4-{[6-(cyclohexylmethyl)pyridine-2-carbonyl]amino}-3-[(4-fluorophenyl)amino]benzoic acid | C26 H26 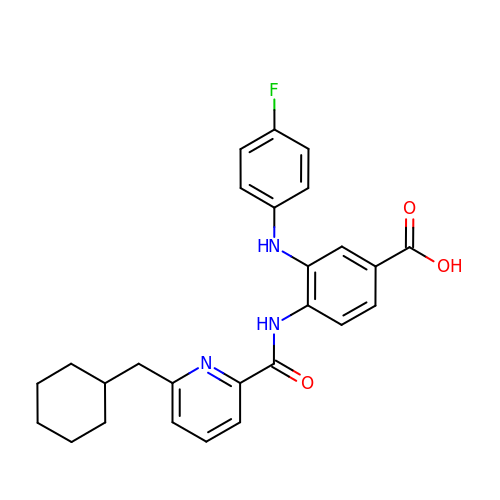F N3 O3 | SFADKDAZWJBQLI-UHFFFAOYSA-N>MPEIVDTCSLASPASVCRTKHLHLRCSVDFTRRTLTGTAALTVQSQEDNLRSLVLDTKDLTIEKVVINGQEVKYALGERQSYKGSPMEISLPIALSKNQEIVIEISFETSPKSSALQWLTPEQTSGKEHPYLFSQCQAIHCRAILPCQDTPSVKLTYTAEVSVPKELVALMSAIRDGETPDPEDPSRKIYKFIQKVPIPCYLIALVVGALESRQIGPRTLVWSEKEQVEKSAYEFSETESMLKIAEDLGGPYVWGQYDLLVLPPSFPYGGMENPCLTFVTPTLLAGDKSLSNVIAHEISHSWTGNLVTNKTWDHFWLNEGHTVYLERHICGRLFGEKFRHFNALGGWGELQNSVKTFGETHPFTKLVVDLTDIDPDVAYSSVPYEKGFALLFYLEQLLGGPEIFLGFLKAYVEKFSYKSITTDDWKDFLYSYFKDKVDVLNQVDWNAWLYSPGLPPIKPNYDMTLTNACIALSQRWITAKEDDLNSFNATDLKDLSSHQLNEFLAQTLQRAPLPLGHIKRMQEVYNFNAINNSEIRFRWLRLCIQSKWEDAIPLALKMATEQGRMKFTRPLFKDLAAFDKSHDQAVRTYQEHKASMHPVTAMLVGKDLKVD[3x]

Leukotriene A4 hydrolase (LTA4H) is a zinc metalloenzyme that stands out with unique dual functionalities that include peptidase activity in addition to lipid metabolism. As an epoxide hydrolase (EH), LTA4H converts leukotriene A4 (LTA4) to leukotriene B4 (LTB4). As an aminopeptidase (AP), LTA4H hydrolyzes natural ligands such as dynorphin, enkephalin, and the tripeptide proline-glycine-proline (PGP), of which PGP has garnered significant interest. Therefore, bi-functional EH and AP activities undergird the intricate pro- and anti-inflammatory regulation, respectively, exerted by LTA4H.

As shown in the M1 metallopeptidase HEXXH-(X)18E motif, the Zn2+ ion was coordinated with H295, E296 H299, and the carboxylic acid side chain oxygen atom of E31826. The OPB-Pro was bound in the AP active site with its prolyl carbonyl group interacting with the zinc atom. Hydrogen bonding interactions were present between the Oε1 atom of Q136 and the Cγ atom of OPB-Pro. Our interpretation is that the Q136 side chain maintains the catalytic water molecule interaction with E296 while simultaneously engaging in multiple hydrophobic interactions via its rotational freedom. The loss of water molecules could afford more favorable binding entropies for nonpolar ligand binding, provided steric clashes are avoided. Also, the structural data suggest that nonpolar ligands are likely necessary for enhancing the peptidase activity due to more favorable binding entropies in the active site. Hence hydrophobic interactions and steric considerations are the primary factors influencing what modified kinetics may be possible.3-methoxy-N-[5-[(3-methylphenyl)sulfamoyl]-1,3,4-thiadiazol-2-yl]benzamide | C17 H16 N4 O4 S2 | 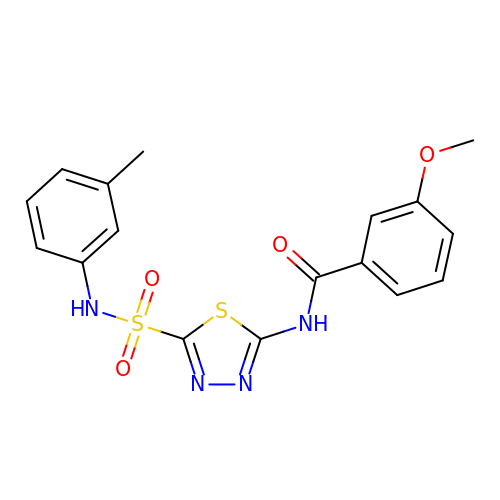NAATWMSNCJQUAW-UHFFFAOYSA-N> MRGSHHHHHHGSIEGRMEKINYLLPEESAEMTLNQVKSLRQIEGRLRKLFSLKNYQEVMPPSFEYTQLYTALESNGKTFNQEKMFQFIKHEGQSITLRYDFTLPLVRLYSQIKDSTSARYSYFGKIFRKEKRHKGRSTENYQIGIELFGESADKSELEILSLALQVIEQLGLNKTVFEIGSAKFFQRLCQLADGSTELLTELLLKKDLSG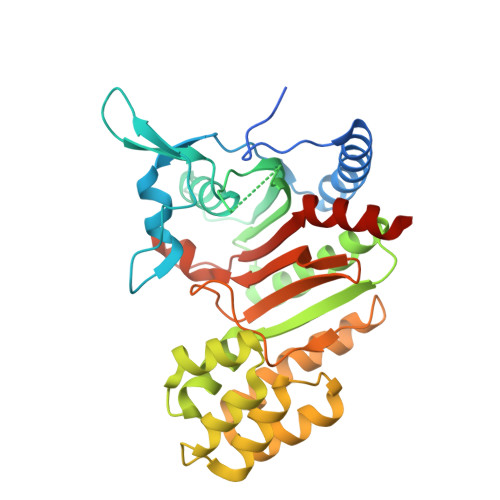LNAFIEKNNFSKELRGLLKEIFITNELSRLENLVTNTKDDVLISSFDQLKEFSEKLSMIKPIIIDLGMVPKMDYYTDLMFKAYSSAANQPILSGGRYDQLLSNFQEEAFAIGFCCHMDTILKALERQELEEDND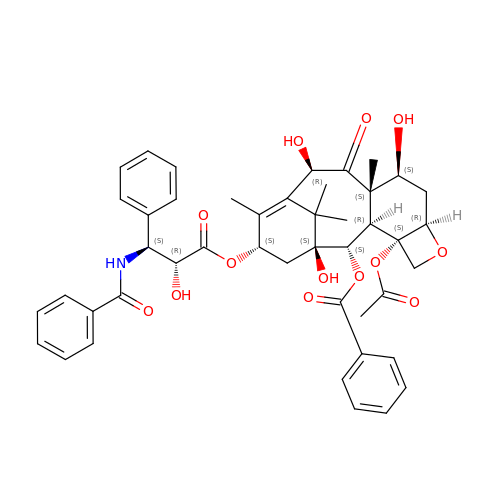Deacetyltaxol | C45 H49 N O13 | TYLVGQKNNUHXIP-MHHARFCSSA-N D-MANNITOL | C6 H14 O6 | 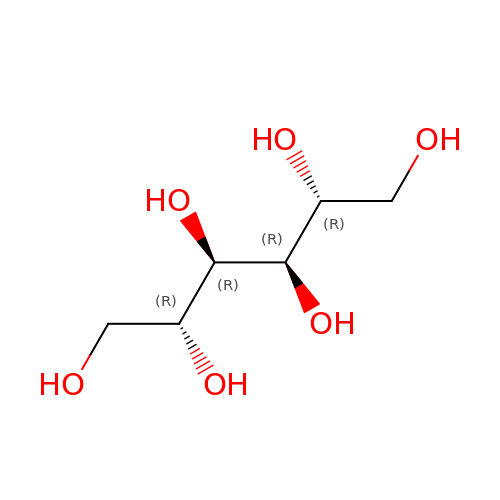FBPFZTCFMRRESA-KVTDHHQDSA-N> MADNMTTTQIEVGPGATNATINFEA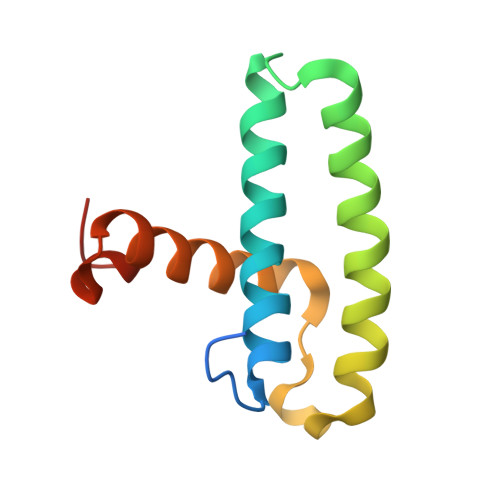GILECYERFSWQRALDYPGQDRLHRLKRKLESRIKTHNKSEPENKRMSLEERKAIGVKMMKVLLFMDPSAGIEGFEPY Putative tumor suppressor ALDH1L1, the product of natural fusion of three unrelated genes, regulates folate metabolism by catalyzing NADP+-dependent conversion of 10-formyltetrahydrofolate to tetrahydrofolate and CO2. The protein exists as a homotetramer, with each 902 amino acid-long protomer organized in three distinct functional domains. Overall, in the ALDH1L1 catalysis, the 4′-PP arm of the Int domain transfers the formyl group cleaved from 10-fTHF in the folate-binding Nt domain to the Ct domain, where it is oxidized to carbon dioxide. Remarkably, the tetrameric state of ALDH1L1 is indispensable for catalysis because the intermediate domain transfers formyl between the catalytic domains of different protomers.

To elucidate the potential effect of NADP+ on the structural organization of ALDH1L1, we also prepared cryo-EM grids after adding 1 mM NADP+ to the full-length protein. Single-particle analysis of the new dataset containing 202,398 particles produced a 2.9-Å resolution map. The arrangement of the Ct core and Int domains in this structure was identical to that in the ligand-free protein and corresponded well to the configuration of the Ct and Int modules revealed by NS-EM. We found that the cryo-EM structures of ligand-free and NADP+-bound ALDH1L1 were highly similar (r.m.s.d. = 0.86 Å). A small difference was observed in the NADP+-binding site, where the C-terminal end of the helix formed by residues 652–666 was better ordered in the presence of the coenzyme. Only the AMP portion of bound NADP+ was clearly visible in the cryo-EM map, while there was no density for the rest of the cofactor. To determine the fraction of free (not occupying substrate entrance tunnels) Int domains, we performed local 3D classification within a mask encompassing each Int domain and calculated the total number of particles that contributed to empty versus occupied classes. This analysis produced estimated average occupancies of 76% and 83% for the Int domain in the ligand-free and NADP+-bound structures, respectively. Instead, the Int domain of chain A was docked at the substrate entrance tunnel of the Ct domain of chain C, whereas the Int domain of chain C was paired to the Ct domain of chain A. Therefore, each Int domain of ALDH1L1 is paired to a Ct domain of the opposite dimer. The 4′-PP group covalently linked to serine 354 of the Int domain was found in the fully extended conformation, penetrating deep into the substrate entrance tunnel of the Ct domain and making multiple contacts with residues forming the tunnel.

>MKIAVIGQSLFGQEVYCQLRKEGHEVVGVFTIPDKDGKADPLGLEAEKDGVPVFKFPRWRARGQALPEVVAKYQALGAELNVLPFCSQFIPMEVINAPRHGSIIYHPSLLPRHRGASAINWTLIHGDKKGGFTIFWADDGLDTGDLLLQKECEVLPDDTVSTLYNRFLFPEGIKGMVQAVRLIAEGTAPRCPQSEEGATYEGIQKKETAKINWDQPAEAIHNWIRGNDKVPGAWTEACGQKLTFFNSTLNTSGLSTQGEALPIPGAHRPGVVTKAGLILFGNDDRMLLVKNIQLEDGKMMPASQFFKGSASSSLELTEAELATAEAVRSSWMRILPNVPEVEDSTDFFKSGAASVDVVRLVEEVKELCDGLELENEDVYMATTFRGFIQLLVRKLRGEDDESECVINYVEKAVNKLTLQMPYQLFIGGEFVDAEGSKTYNTINPTDGSVICQVSLAQVSDVDKAVAAAKEAFENGLWGKINARDRGRLLYRLADVMEQHQEELATIEALDAGAVYTLALKTHVGMSIQTFRYFAGWCDKIQGATIPINQARPNRNLTLTKKEPVGVCGIVIPWNYPLMMLSWKTAACLAAGNTVVIKPAQVTPLTALKFAELTLKAGIPKGVVNILPGSGSLVGQRLSDHPDVRKIGFTGSTEVGKHIMKSCALSNVKKVSLELGGKSPLIIFADCDLNKAVQMGMSSVFFNKGENCIAAGRLFVEESIHNQFVQKVVEEVEKMKIGNPLERDTNHGPQNHEAHLRKLVEYCQRGVKEGATLVCGGNQVPRPGFFFQPTVFTDVEDHMYIAKEESFGPIMIISRFADGDVDAVLSRANATEFGLASGVFTRDINKALYVSDKLQAGTVFINTYNKTDVAAPFGGFKQSGFGKDLGEAALNEYLRIKTVTFEY[4x]> SASRDDWRAARSMHEFSAKDIDGHMVNLDKYRGFVSIVTNVASQCGKTEVNYTQLVDLHARYAERGLRILAFPSNQFGKQEPGSNEEIKEFAAGYNVKFDMFSKIEVNGDDAHPLWKWMKIQPKGKGILGNAIKWNFTKFLIDKNGVVVKRYGPMEEPLVIEKDLPHYF;> XCRVDLQGW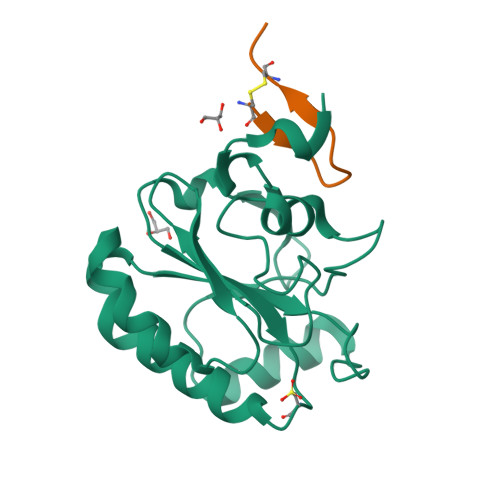RRCRRX>[4x]MNNSFLDKLIETKELKNSLYNVLKHNFLYHSNKIEGST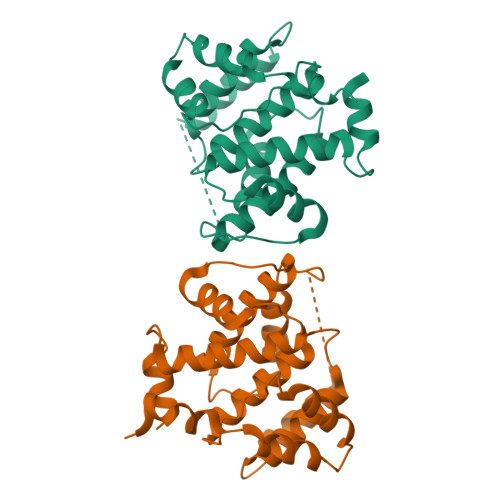FTTEALALLLDKNVVTGRHTLDDVQETVNSSYVFDTVIDSLKEKITHNFLRNLHSSLIFNTTLHSRGMAGIYKTIPNMILGTDVSIAQPFEVEPKLDELIEWYYSQSEVSIKVIAEFHYRFELIHPFQDGNGRIGRFVMLKQMLENNLPIKIVSWDSEDLYRNSLNSCSLGNYVPLIEYLSSLEDFREVYKMLWKLE4-[4-(naphthalen-1-ylmethyl)piperazin-1-yl]-4-oxobutane-1-thiol 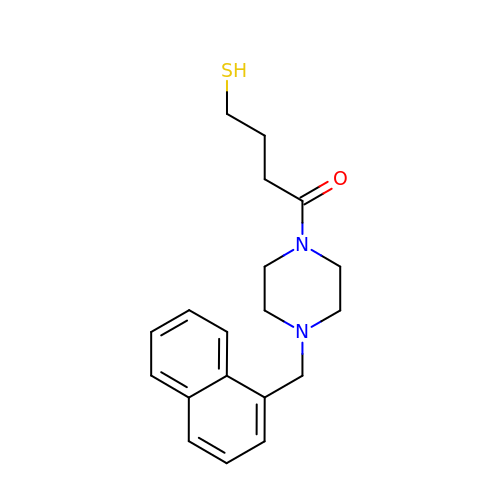| C19 H24 N2 O S | KGVPRVVVECAVEV-UHFFFAOYSA-N N-[(5R)-1,1-dioxo-2,3,4,5-tetrahydro-1H-1lambda~6~-benzothiepin-5-yl]-2-hydroxyquinoxaline-6-carboxamide 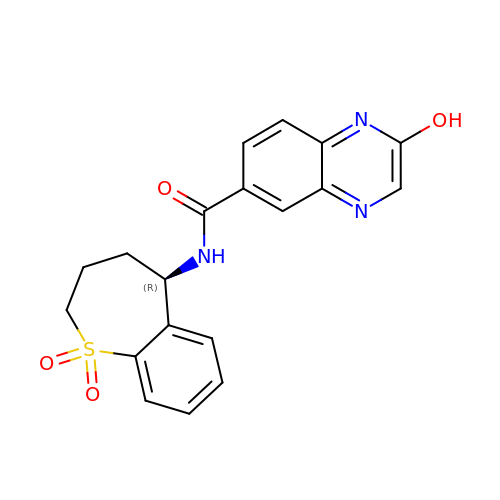| C19 H17 N3 O4 S | DYZHGISSMYNBJE-CQSZACIVSA-N> MGLLSLIRGLKKKEGEARILVLGLDNAGKTTILKALSEEDITTITPTQGFNIKSLSRDGFNLKIWDIGGQKSIRPYWRNYFDQTDALIYVIDSADSKRLSESEFELTELLQEEKMTGVPLLVFANKQDLVGALAADEIASTLDLTSIRDRPWQIQACSAKQGTGLKEGMEWMMKQVKLEHHHHHH;> GPRKITIALLGLDNAGKTTLLNSIQGEVDRDTTPTFGFNSTTLNEGKYKIEVFDLGGGKNIRGVWKKYLAEVHAIVYVVDAADPGRFEESKMTMAEVLENQFMRDKPICIFANKQDLPTAAPAAEVVKGLGLATCRNSHNVFPCTAKMPAGQDVDHRLRDGLKWLVGTVDREFGRLDPRVQTEAEEVRQEEARKKKEREERLRKQREERLRQQKEEEERAREVEKENELHDGKAPSLLAAGGGVVGAAAAGVNGVMVDEQQEL

The small G-proteins of the Arl family Arl3, Arl6 and Arl13B have been shown to be important in the trafficking of ciliary proteins and structural integrity of the cilium. As most small G-proteins Arl3 cycles between inactive GDP-bound and active GTP-bound forms and in the latter it binds specifically to effectors. Arl13B is an unusual Arl protein containing a C-terminal coiled-coil and proline rich region in addition to its G-domain. Here we describe a molecular function for Arl13B acting as GEF for Arl3 whereby the nucleotide state of Arl13B determines its catalytic activity in this activation cascade.

We thus co-crystallized CrArl13B·GppNHp and CrArl3·GDP in the presence of alkaline phosphatase in order to allow formation of nucleotide free CrArl3. The obtained crystals diffracted to 2.5Å and the structure was solved by molecular replacement showing one complex in the asymmetric unit. Although crystallization was done in the presence of alkaline phosphatase GppNHp was clearly visible in both active sites, suggesting that the structure represents the post-nucleotide-exchange state. The structure shows indeed that a major part of the interaction is mediated by switch I and II of CrArl13B which contact CrArl3 via α4Arl3, β6Arl3, and α5Arl3 located opposite to the nucleotide binding site. Further interactions are between the long α-helix α6Arl13B which makes a 90° turn at residue G189, and α3/ α4Arl3. In the crystal structure the nucleotide binding site of CrArl3 is not directly contacted by CrArl13B. We were not able to trap the interacting residues presumably due to the presence of nucleotide and/or the flexibility of the interacting residues of Arl13B. Considering the length of the C-terminus required for catalysis (see below) it is however suggestive that the mobile C-terminus of Arl13B is involved in the GEF reaction by contacting the relevant surface of Arl3. Switch I mutant CrArl13BF53A showed a markedly decreased GEF activity whereas the D46A, F51A, N75A, and Y83A mutants had only a minor effect. The charge-reversal mutations K210E/R216E in α6Arl13B as well as D103R and D146R in CrArl3 show no activity, as expected, whereas a control mutation H154W outside the interface has no effect. In support of their importance residues 212–228 are highly conserved among species and we would speculate that these residues contact Arl3 close to the nucleotide binding site.(3R,4R,5R)-3-hydroxy-5-(hydroxymethyl)piperidin-4-yl 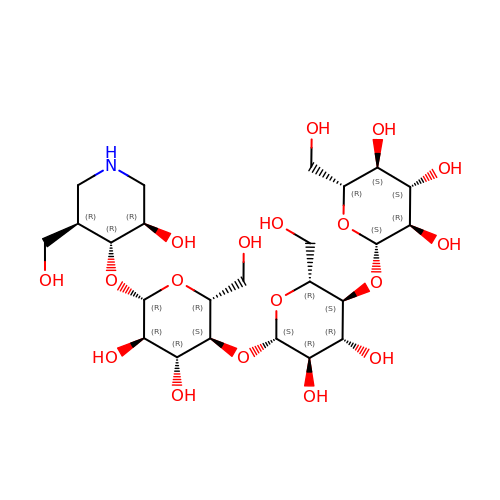beta-D-glucopyranosyl-(1->4)-beta-D-glucopyranosyl-(1->4)-beta-D-glucopyranoside | C24 H43 N O18 | WWLNURYAWFMUKB-QPKZCLDCSA-N>AKGNDSKDFNNSYGISHITRDNMVKIPQQQNSDQFKVPAFDESTIKNIASAKGKNASGNTIDLDVWDSWPLQNADGTVATYHGYQIVFALAGDPKDSNDTSVYLFYKKAGDKSIDSWKNAGRVFKDSDKFVPNDPHLKNQTQEWSGSGTLTKDGKVRLFYTDYSGKQYGKQTLTTAQVNMSQPNDNTLKVDGVEDYKSIFDGDGKIYQTVQQFIDEGGWDTGDNHTLRDPHYIEDNGHKYLVFEANTGTEDGYQGEDSLYNRAYYGGNNPFFQSEKKKLLEGSNKEKASLANGALGIIELNDDYTLKKVMKPLITSNTVTDEIERANIFKKDGKWYLFTDSRGSKMTIDGIGQDDVYMLGYVSNTLTGKYKPLNDTGLVLHMDLDP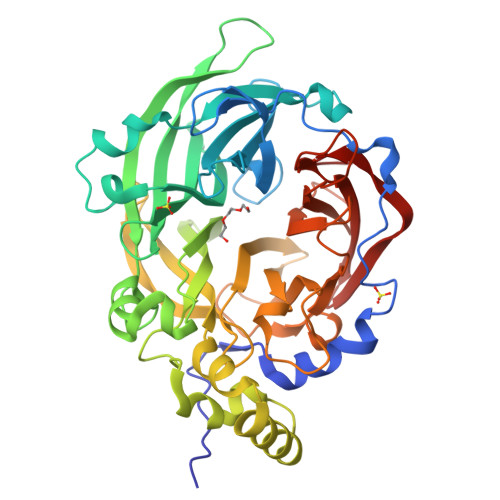NDKTFTYSHFAVPQTKGDNVVITSYMTNRGFYEDNHSTFAPSFLVNIDGSKTSVVKDRVLEQGQLTVDED[4x]3-SULFOOXY-1H-INDOLE | C8 H7 N O4 S | 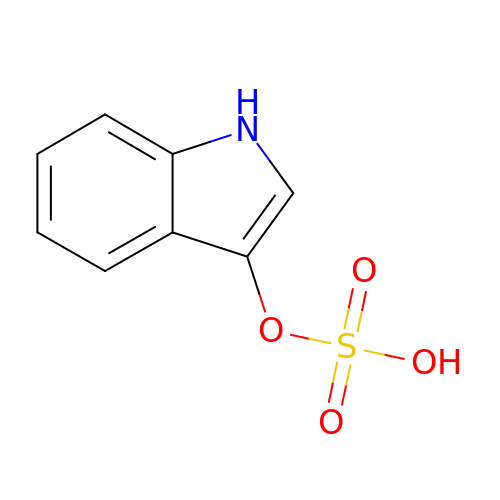BXFFHSIDQOFMLE-UHFFFAOYSA-N> MNDVKVIKLSGSLGRRFGVFHRYAVDSYPEAIRALSSQVDGFKEYMQSEVGSRSKFAIFVDGVNVGHHEEEKFKCAKEIRIVPIPTGSKTGGLFQVVLGAAIMVAAFYTGGASLALMGTMSSSLFMMGGAMVLGGVMQMISPQPGGANFEVQSSKNKPSYAFGGAVNTTAAGYPLPVPYGYRAGGGATFSAGSYAEDMS;> MVDKVAGLSLDVDVSTVQRAVKSLKEFSKANDQAADSMGSLINESEVAKQKAKEHAEQLRRQRKEYEAVEKAIDPTVSKMERLKIASQQLDKLWQQGVVPDETFFRLGEMLDLQNAKLARSRAMLTEEGQAALQEAKAKEQAAVRSKAFMDALNGQVNAIGKTHAELMELKAAELGLSKEAAPLIAKLKDQGRAMNAAGISAGEYRQAMRMLPAQITDVVTSLASGMPVWMVAIQQGGQIKDSFGGIGNTFKVLLSYINPVTAGVGVLVGSLGILAKAGYDSYKSITDIQNALIETGGYAGVTAEELDSVSKKIAQTSNSTIGSIREIVTELASSGKYTREQIQNITKATAEWSASTGKSASQIISEFEKIASDPVKGLKKLNEQYNFLEKGQLTYIDTLSRTKGETEAVSEATKLFADVMEKRMKSIADNATPLEKMWSDIKQWASDAWGWVGDHTLGALNLIIDVVQGTVIQVKMILAKGDEYISNFIASAIKATQSLPGMSDFGADVLKEQENIVKSSRDNYDQLASDLDAINARVEKGEMGYIEAMRQRRTLEKQYSEETKEAIRKEAEEIEKRNRERNKQSKIVRSPTEQFDKELISLRAQLKVLQEHKEIGQKLSAQRKALFTTEATIAVLREASSKRQLSAEEKALLASQERVIELAKQKAEIGDQIVKQQQLNDLTDKSLKFVNEMTAATEQLNASRGLSTRDMERQAELAKITTDYINSGGSEGDEKLQNMIKAQNDYYAAEDAKRADWLAGAESAFADYGDAAMDMYGNVNEIASSALNGMSDMMVQFLTTGKANFEDFAKNIIGMIIKMIAQMVIFNTISGMMGGKTWSFAGGASSGASAASQATPTPAASVFRSVSSGGAAVSLAAAAGSVATSGFNASNSAPKVVNHSGGGTVVDVSGMEVKVDNGSDPRGISQGVEMMFKKMIRESCSQGGEVYNYIQEKTGG;> MATLDTFGWCTQVQGGGGSLTTTNSDRSIQFGNGYMQLASSGFNTTRREYSVVYAGEDFMAVYDFCNSHRIKPFAWTPPDGKIGIWVVKPNSLGAKPVSRDVMEINVTFMEQFTSME;> MSENKKLYDEESGKSLFHNCLQSLYPGEIITLIEVDGSKFGAQVYRFHGENIQYTPEEIMQAQQTGTLPPKEITFRGEKYGARPFGISGISFDSSGKATKPQLTVANIDSRVSAMIRAYNGLMQAKVTIWITQRELINSDGSIADGAYRKLVYYIERPNYVDKSVARFDLTSPYDMDGIMIPSRLTQSVCYFAQRGWYKTGKGCGYNGQNGYFDKDNNPVDDPSLDFCPGTVTACRLRFGANNELDFGGCAVASLQRKNQ;> MIQKVISGSKGGSQKPHNPVEMEDNLISINKIKILLAVSDGEIDETFSLKQLMFNSVPVQNEDGSFNFEGVKAEFRPGTQTQEYIKGMEDSSSEVTVNREVTTDNPYTISVTNKTLSAIRIKMFMPRGVRIESNGDKNGVRVEYEVQQAVDGGSFETVLTDVIEGKTMSGYDRSRRVNLPNFNNQVIFRVVRKTPDSNDSNVVDAIQVKSYAEVIDAKFRYPLTGLLFVEFDSKMFPNQLPTISIRKRWKIVNVPSNYDPESRTYNGNWDGTFKKAWTNNPAWVLYDLMINQRYGLDQKELGIAVDKWALYEAAQYCDQMVPDGKGGTEPRYLCDVIIQSQTDAYKVIRDICSIFRGMSFWNGESISVIIDRPREPAYIFTNDNVVNGDFSYTFASEKSMYTTCNVMFDDEQNMYQQDVEPVFDREATLRFGNNVTSITAIGCTRRSEANRRGRWILKTNLRSTTVNFATGLEGMIPTIGDVVAIADNFWSSNLTMNLSGRLLEVSGSQIFLPFRVDARAGDFIIVNKPDGKPVKRTISSVSADGKTIEVNIGFGFPVKPNTVFAIDRTDIALQQYVVTKIDKGDDDEEFTYKITAVEYDPNKYDEIDYGVNIDDRPTSIVEPDQIPRPKNVQVSSESRIVQGMSVETMIVSWDKVPYAVFYDVQWRKDNGNWQNVPQTANKEVYVEGIYAGNYQVRVRSVAGSGTTSGWSNIVAATLTGKQGEPGRPINLTATDDVVFGIRTKWGFSDGSGDTAYTELQQSPDGTVDNASLLSLIPYPQHEYYHSPMPGGNIVWYRVRTVDRIGNVSQWTDFVRGMASTNVDDIIGEISVDIENSPGYEWLVDNATDNAAQNSANAEAAIENALANDKDAIYMKKENGKRKAEYTKSLKLIADETQARVTAIEQLKASFGDQISASNSELREVIATETEALSREIDQLKAQIGDDIQASLTDIREVIATETEALSREIDQLKAQIGDDIQASLTDIREAIANETEARTQADLTLSARLGNNEAALAQKLDSWSNADSTGAMYGVKLGLKYNGQEYSAGMAMSLVGSGAAVKAQILFEASRFAIMTGMNGQTQYPFVVENGQVILSSAIIKNGFITNAMIGNFIQSNNYVFNQSGWRLDKGGTFENYGSDGEGAMKQTNTTISVRDASGRLRVQIGRLTGSW

Siphophage T1 is representative of the T series of model Escherichia coli phages, which has been observed to infect not only sensitive strains of E. coli but also some strains of Shigella dysenteriae. Siphophages possess a long, flexible, and non-contractile tail that plays a crucial role in host recognition, cell envelope penetration, and DNA injection. Connected to the head through a connector complex, the tail of a siphophage consists of three main components: a tail tube, a tape measure protein (TMP), and a distal tip. Using cryo-EM, we resolved the three-dimensional (3D) structures of the icosahedral head, head–tail complex and the tail tip of a laboratory-adapted fiberless mature T1 at resolutions of 3.5 Å, 3.6 Å, and 4.3 Å, respectively.

The distal tip of T1, which is cone-shaped and assembled by proteins gp33, gp34, gp36, gp37, and gp38, displays structural similarity to that of phage lambda. In combination with alphaFold3, we also obtained all atomic models of the tail tip, including the distal tail protein gp37, the hub protein gp36, the central fiber protein gp33, the insertion protein gp34, and the C-terminus of TMP gp38. The structure of the cone-shaped distal tail tip of T1 is highly similar to that of phage lambda. In particular, the features of the T1 tail tip, which are essential for infection, trans-membrane and DNA ejection, are structurally conserved across the widespread lambda-like siphophages with the cone-shaped tip, thus suggesting that T1 is another representative of lambda-like siphophages. Furthermore, structural comparisons of the tail tip among T5, DT57C, Chi, lambda and T1 reveal that with the exception of the conserved and essential structural components of the inverted tip formed by the distal tail protein, hub, and central fiber protein, etc., a variety of add-on components diversify the inverted tip decorated with different lateral fibers, receptor-binding proteins or collars, etc. For instance, the distal tip of T5 and DT57C transform from a triple bifurcation to an extended β-helix structure, while the distal tip of T1 forms a long and flexible α/β-helix fold structure. During infection, the tail tip penetrates the cell envelope. However, whether the tip of T1 is curved during the infection still needs to be further studied.> MRKRVVVTGVGAIHPDGNDVTAIKSKVIQKLLGQESKNNTTASSIIRTLSDFDGAKYINNRLRRKIDEFSVYGIVAVEMA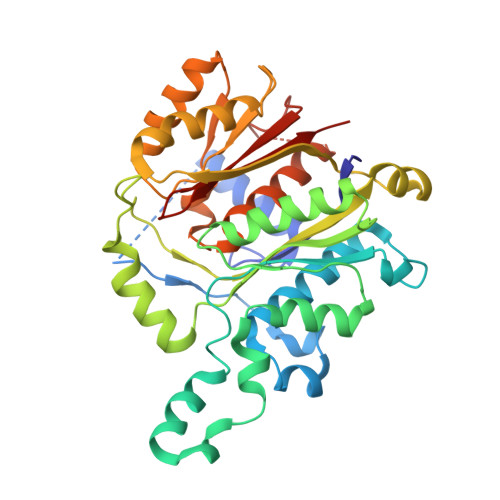LKASRLDVDKLDPNRVGIYVGNCFGGWQHIEDEVKALHIEGIKGMGPYVATAWFPAALQGQLSLLYGFSAQSKTFSTSDVAGMQAIGYAAEAISNGVAEVMLCGASEHLSSPLVKNLLEKTSSQKHSEVFGEKQPGDFSEGAAFLVLEERQHALERGASILCELTGFVDYFAPDKNTRNNTLEYTAELFNHNENAVFIMDGIYDDEKEITSKAFSNKEIKTSFINLRPYLDNQFSVSGVIDSVLASSFLSESHGDEEQQSKKINEFSNTNQIIIQRFSNQGHVCALSFSAI> SEESQAFQRQLTALIGYDVTDVSNVHDDELEFTRRGLVTPRMAEVASRDPKLYAMHPWVTSKPLPEYLWKKIANNCIFIVIHRSTTSQTIKVSPDDTPGAILQSFFTKMAKKKSLMDIPESQSEQDFVLRVCGRDEYLVGETPIKNFQWVRHCLKNGEEIHVVLDTPPDPALDEVRKEEWPLVDDCTGVTGYHEQLTIHGKDHESVFTVSLWDCDRKFRVKIRGIDIPVLPRNTDLTVFVEANIQHGQQVLCQRRTSPKPFTEEVLWNVWL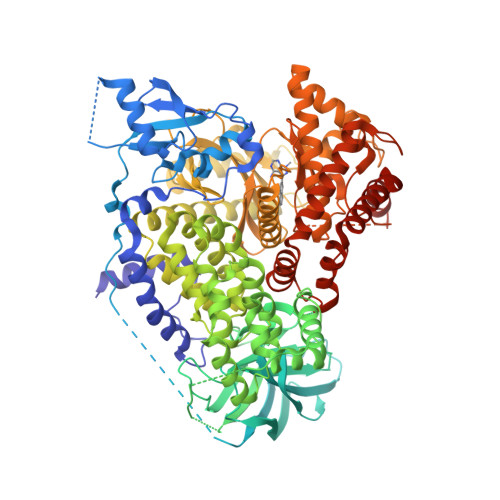EFSIKIKDLPKGALLNLQIYCGKAPALSSKASAESPSSESKGKVRLLYYVNLLLIDHRFLLRRGEYVLHMWQISGKGEDQGSFNADKLTSATNPDKENSMSISILLDNYCHPIALPKHQPTPDPEGDRVRAEMPNQLRKQLEAIIATDPLNPLTAEDKELLWHFRYESLKHPKAYPKLFSSVKWGQQEIVAKTYQLLARREVWDQSALDVGLTMQLLDCNFSDENVRAIAVQKLESLEDDDVLHYLLQLVQAVKFEPYHDSALARFLLKRGLRNKRIGHFLFWFLRSEIAQSRHYQQRFAVILEAYLRGCGTAMLHDFTQQVQVIEMLQKVTLDIKSLSAEKYDVSSQVISQLKQKLENLQNSQLPESFRVPYDPGLKAGALAIEKCKVMASKKKPLWLEFKCADPTALSNETIGIIFKHGDDLRQDMLILQILRIMESIWETESLDLCLLPYGCISTGDKIGMIEIVKDATTIAKIQQSTVGNTGAFKDEVLNHWLKEKSPTEEKFQAAVERFVYSCAGYCVATFVLGIGDRHNDNIMITETGNLFHIDFGHILGNYKSFLGINKERVPFVLTPDFLFVMGTSGKKTSPHFQKFQDICVKAYLALRHHTNLLIILFSMMLMTGMPQLTSKEDIEYIRDALTVGKNEEDAKKYFLDQIEVCRDKGWTVQFNWFLHLVLGIKQGEKHSA>MNTVESRPVSVLFLCTGNTARSQLAQVLLEHHGGGRYAVTSAGLEPGSVNPLTVQVLQESGLPTGHLQAKGVRPLIAEHFTYVITVCDRAEANCPIFPNATYRLHWPFEDPAAATGSEEERLAVFRHVRDEIDARIQAWVAARV[2x]

D. indicus contains the typical arsRBC operon that encodes two regulatory proteins (ArsR1 and ArsR2), two arsenate reductases (ArsC2 and ArsC3) and an arsenite efflux pump protein (ArsB). In order to explore the difference between the two species, D. radiodurans and D. indicus, to the arsenate resistance we analyzed the arsenate reductases that belong to the ars operon, which are able to convert As(V) into As(III). DiArsC2 structures are composed of an α/β domain and four parallel β-strands which are flanked by three helices and two small helices. The reduction mechanism of arsenate involves three cysteines, Cys15, Cys87, and Cys94.

Thus, we undertook the structural studies of DiArsC2 and we were able to crystallize two different forms of the enzyme: native (DiArsC2) and bound to arsenite (DiArsC2-As). The crystal structures of DiArsC2 and DiArsC2-As were determined and refined at resolutions of 1.65 and 1.50 Å, respectively. In the case of the DiArsC2-As structure, a disulfide bridge between Cys87 and Cys94 is formed. Although the protein was co-crystallized in the presence of arsenate (AsO43−), the density observed close to the catalytic Cys15 suggests the presence of AsHO32−. This molecule is located in a positively charged pocket and establishes a network of hydrogen bonds with the main-chain nitrogen atoms of residues G17NTARS22, Thr16 and Ser22 hydroxyl and Arg21Nε groups, as well as water molecules. Moreover, the arsenate is located in a positive-charged pocket which is accessible from the external environment. The DiArsc2-As structure represents the final stage, where Cys15 is bound to As(III), however the ligand cannot be released since Cys87 forms a disulfide bridge with Cys94. Since in our DiArsC2 structure the disulfide bridge between these two residues is not formed (at least in chain B, where density is observed) this could indicate that an As(V) reduction event already took place in the DiArsC2-As structure, leading to the formation of the Cys87 – Cys94 disulfide bridge. The lack of mobility of the PTPase loop (where Cys15 is located) together with the high flexibility of the loop that contains Cys87 and Cys94 suggests that Cys87 is the residue responsible for the release of As(III) bound to the Cys15. In fact this loop is readily accessible by the thioredoxin reductase system to reduce the Cys87 – Cys94 disulfide bridge and allow a new As(V) reduction cycle to occur.> NADDQLKQLSALEGANGYVIF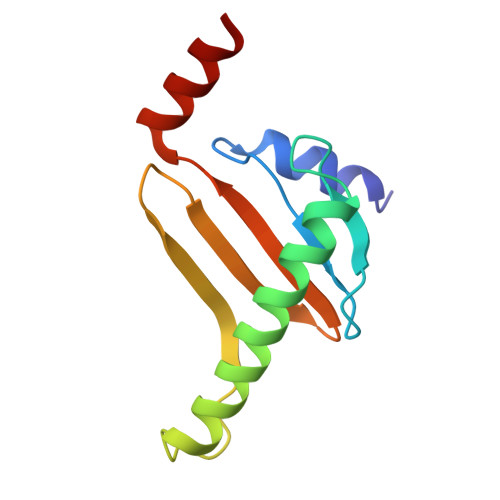NESGIPLKRHEKSISHEKAVHIAALVSDLWNVSKKVIQRDLKTPENDIEVIRLRTKHSYEYIITQSGDFTMLAIQLCGKAIEEAKKAAA> MWHSDDLDDLLGSHHHHH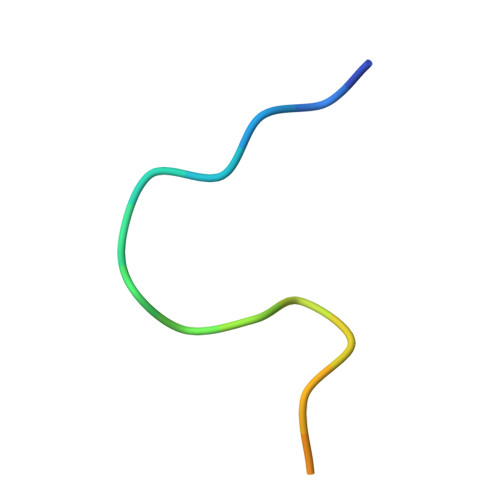H> GPDMNNELHNENTIRILISSDPHVGYGEKDPVRGNDSFVSFNEILEIARERDVDMILLGGDIFHDNKPSRKALYQALRSLRLNCLGDKPCELELLSDTSLTTGDTAVCNINYLDPNINVAIPVFSIHGNHDDPSGDGRYSALDILQVTGLVNYFGRV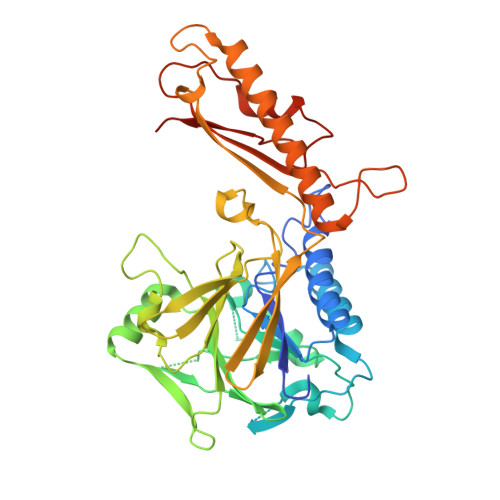PENDNIVVSPILLQKGFTKLALYGISNVRDERLYHSFRENKVKFLRPDLYRDEWFNLLTVHQNHSAHTPTSYLPESFIQDFYDFVLWGHEHECLIDGSYNPTQKFTVVQPGSTIATSLSPGETAPKHCGILNITGKDFHLEKIRLRTVRPFIMKDIILSEVSSIPPMVENKKEVLTYLISKVEEAITEANAQWYEAQGTVPVVENEKPPLPLIRLRVDYTGGYQTENPQRFSNRFVGRVANATDVVQFYLKKVDENLYFQ>[2x]MKKRILAVAVTSMLLSASVFAQETVVPSRVGDLKFESDFPTQETMKNMLNEMDFQRATQAYLWGIPASSIMEWLNVSRNDFKFEEGQMGFFNTLKQKQGIITANFTTPYVIGTWNLEKTGPLIINLPEAKMAGMMLDVHQRVLSDLSLLGPDKGKGGKYLIVPPGEKYKDLNPKGYYVIRPKTNVVYGGIRILEPDVDRVVKQVV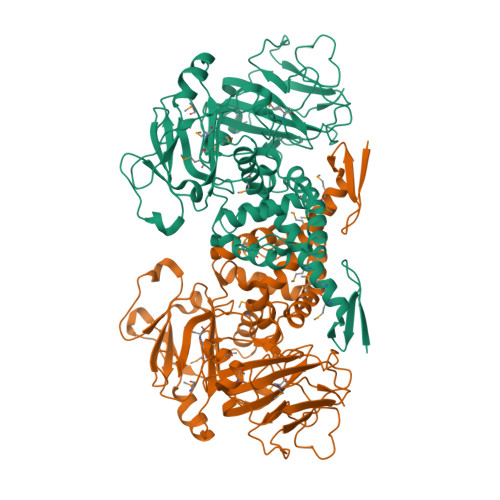PNITTQPYADGKLGRKIPVAQVPEIDWTHIPKDGLEYWKTIHQIIQENPVEERDRFVMAQLKFLGIEKGKPFNPTEEQKKILLEASKVGRAMAQSNDYTKRFTQPYWKGTNWKDAISVSLDQRSENYDELDERAAWFYEAITVSRGMKSTIPGFGQRYLVTYQDSDGNWLSGEHTYKLHVPANVPASNFWSTTVYDENNRLMIINDAGSPDISSRKNLKVNSDGSIDVYYGPKPVKGYENNWVQTNPGEGWFTYFRFYGPTEKMFDKSWTMGDIELVKLEHHHHHH>GDKEGKTGEVQTLTEKIEEAGMPDHVKETALKELNRYEKIPSSSAESSVIRNYIDWLVALPWTDETDDKLDLKEAGRLLDEEHHGLEKVKERILEYLAVQKLTKSLKGPILCLAGPPGVGKTSLAKSIAKSLGRKFVRISLGGVRDESEIRG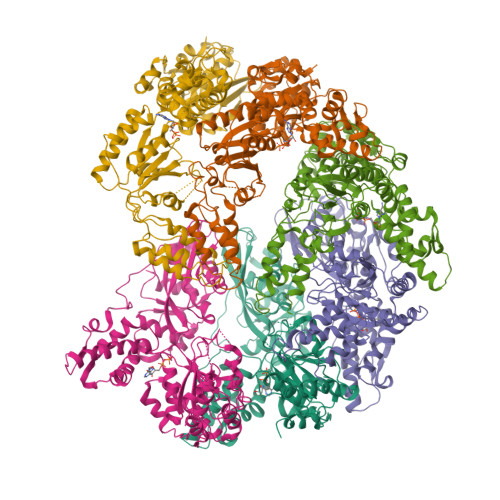HRRTYVGAMPGRIIQGMKKAGKLNPVFLLDEIDKMSSDFRGDPSSAMLEVLDPEQNSSFSDHYIEETFDLSKVLFIATANNLATIPGPLRDRMEIINIAGYTEIEKLEIVKDHLLPKQIKEHGLKKSNLQLRDQAILDIIRYYTREAGVRSLERQLAAICRKAAKAIVAEERKRITVTEKNLQDFIGKRIFRYGQAETEDQVGVVTGLAYTTVGGDTLSIEVSLSPGKGKLILTGKLGDVMRESAQAAFSYVRSKTEELGIEPDFHEKYDIHIHVPEGAVPKDGPAAGITMATALVSALTGRAVSREVGMTGEITLRGRVLPIGGLKEKALGAHRAGLTTIIAPKDNEKDIEDIPESVREGLTFILASHLDEVLEHALVGEKKLEHHHHHH[6x]> GKECEFAMRLVPGFNPLRQVDANGKECRGNVELPFCKGYCKTSESGTHGFPPRVQNSKVCTLVTTSTRKVVLDDCDDGADESVKFVMVPHGTDCEC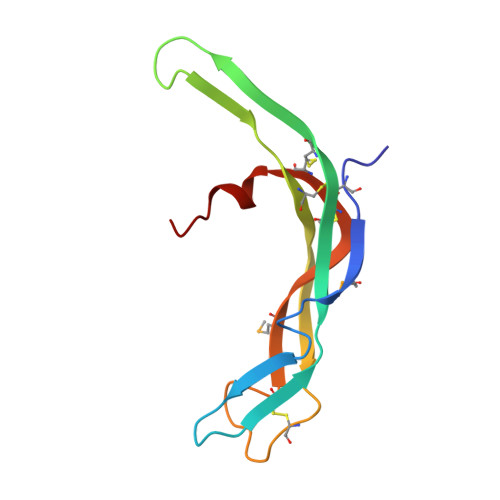SAVPLEQHHS>DICDPNPC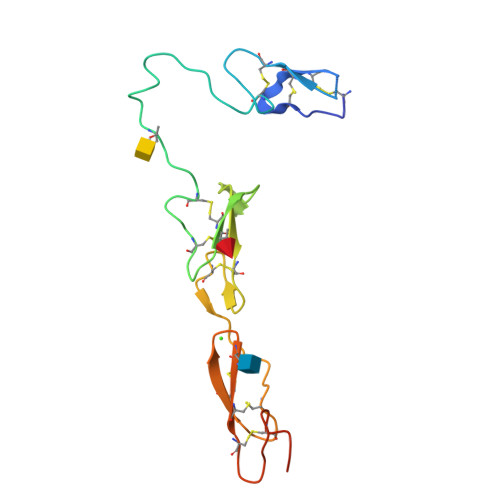ENGGICLPGLADGSFSCECPDGFTDPNCSSVVEVASDEEEPTSAGPCTPNPCHNGGTCEISEAYRGDTFIGYVCKCPRGFNGIHCQHNINECEVEPCKNGGICTDLVANYSCECPGEFMGRNCQYKGGGHHHHHH[2x]> MPAHYISDIAQQREGHEAAADFLDIFSHRLITQYYRIWRKYSYPATFEAGGQDKTSQYLLGLARLGIPGCAQNIATPVSRFLALLPLMLLPGRTAEGLTSLVTLLAPGTQARVWHHDRRRIPLKTPLTMRVHHPVSLKSRPVMGDHATDVNGQVLLQLSTQTGSEVQGWLPGGHLYSDL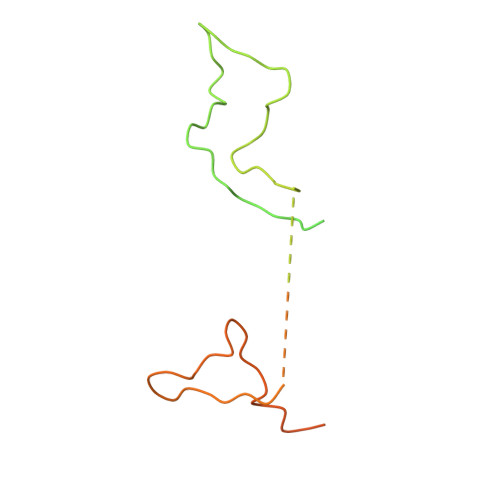LALLHVYLGSRLDVRLQLCVERSLLPDARLSCRPAAGSPQLGRTAVMRTQAKITTSAARVMTISLGRYQRVQEHYQRKETQENGDYRW> SNAMASQIDQYAVFGNPINHSKSPFIHTLFARQTQQSMIYTAQCVPVDGFTEAAKHFFAQGGRGCNVTVPFKEEAYRFADRLTERARLAGAVNTLKKLDDGEILGDNTDGEGLVQDLLAQQVLLKGATILLIGAGGAARGVLKPLLDQQPASITVTNRTFAKAEQLAELVAAYGEVKAQAFEQLKQSYDVIINSTSASLDGELPAIDPVIFSSRSVCYDMMYGKGYTVFNQWARQHGCAQAIDGLGMLVGQAAESFMLWRGLRPGTKQILRELRKNLEGAL;> QIDQYAVFGNPINHSKSPFIHTLFARQTQQSMIYTAQCVPVDGFTEAAKHFFAQGGRGCNVTVPFKEEAYRFADRLTERARLAGAVNTLKKLDDGEILGDNTDGEGLVQDLLAQQVLLKGATILLIGAGGAARGVLKPLLDQQPASITVTNRTFAKAEQLAELVAAYGEVKAQAFEQLKQSYDVIINSTSASLDGELPAIDPVIFSSRSVCYDMMYGKGYTVFNQWA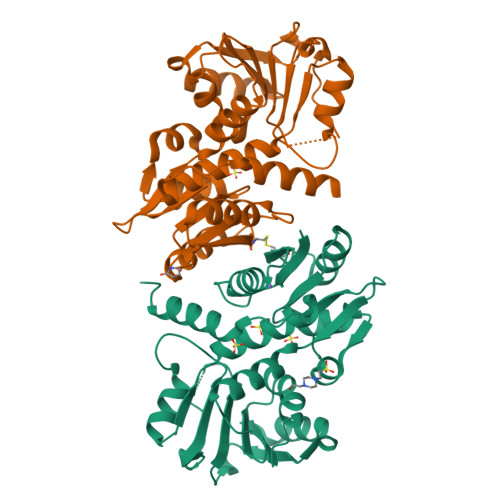RQHGCAQAIDGLGMLVGQAAESFMLWRGLRPGTKQILRELRKNLEGAL4-({3-[2-(dimethylamino)ethyl]-1H-indol-1-yl}methyl)-N-hydroxybenzamide | C20 H23 N3 O2 | 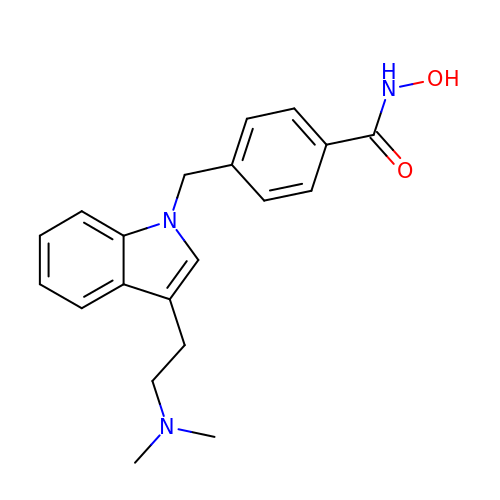OQQDAERWKGMJMN-UHFFFAOYSA-N3-(4-{[(4-fluorophenyl)carbamoyl]amino}-1H-pyrazol-1-yl)-N-(2-methylpyridin-4-yl)benzamide 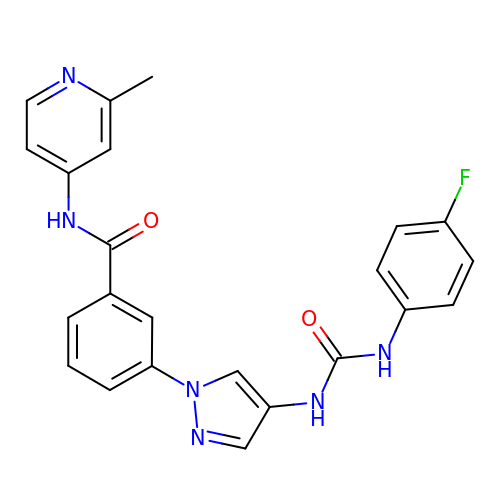| C23 H19 F N6 O2 | CHEAXMFRMQDNIT-UHFFFAOYSA-N> GPMDFLR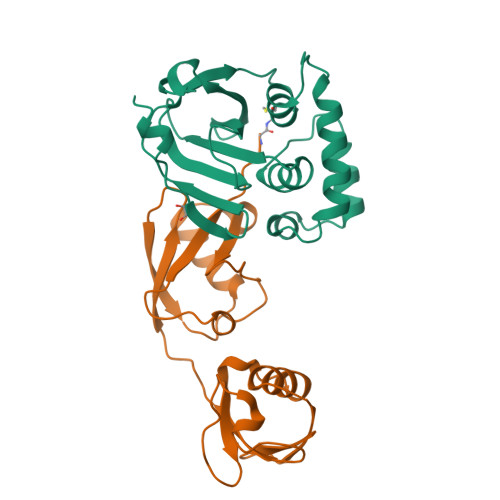SLDWTQVIAGQYVSNPRFNISDYFEIVRQPGDGNCFYHSIAELTMPNKTDHSYHYIKRLTESAARKYYQEEPEARLVGLSLEDYLKRMLSDNEWGSTLEASMLAKEMGITIIIWTVAASDEVEAGIKFGDGDVFTAVNLLHSGQTHFDALRILPQFETDTREAL;> MGWDLTVKMLAGNEFQVSLSSSMSVSELKAQITQKIGVHAFQQRLAVHPSGVALQDRVPLASQGLGPGSTVLLVVDKSDEPLNILVRNNKGRSSTYEVRLTQTVAHLKQQVSGLEGVQDDLFWLTFEGKPLEDQLPLGEYGLKPLSTVFMNLRLRG> GSSGSSGPILELKEKIQPEILELIKQQRLNRLVEGTCFRKLNARR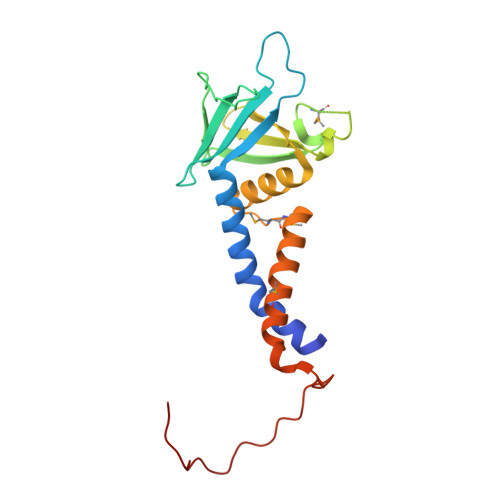RQDKFWYCRLSPNHKVLHYGDLEESPQGEVPHDSLQDKLPVADIKAVVTGKDCPHMKEKGALKQNKEVLELAFSILYDSNCQLNFIAPDKHEYCIWTDGLNALLGKDMMSDLTRNDLDTLLSMEIKLRLLDLENIQIPDAPPPIPKEPSNYDFVYDCN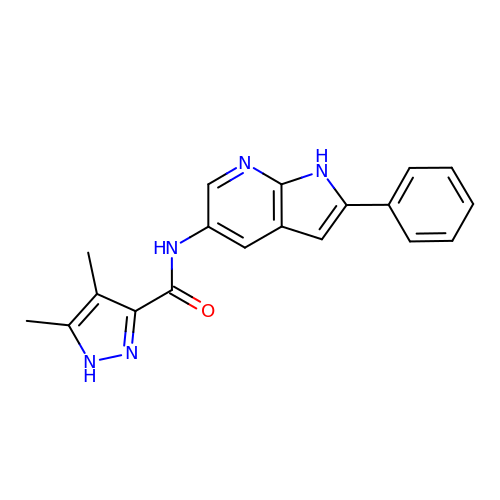4,5-dimethyl-N-(2-phenyl-1H-pyrrolo[2,3-b]pyridin-5-yl)-1H-pyrazole-3-carboxamide | C19 H17 N5 O | NVSHVYGIYPBTEZ-UHFFFAOYSA-N> GELVRTDSPNFLCSVLPTHWRC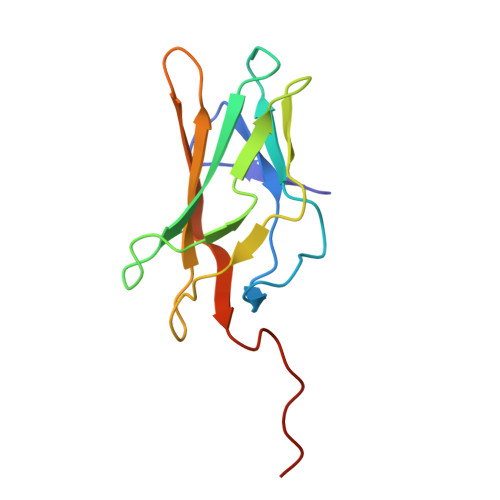NKTLPIAFKVVALGDVPDGTLVTVMAGNDENYSAELRNATAAMKNQVARFNDLRFVGRSGRGKSFTLTITVFTNPPQVATYHRAIKITVDGPREPRRHRQK> MAASGLDHLKNGYRRRFCRPSRARDINTEQGQNVLEILQDCFEEKSLANDFSTNSTKSVPNSTRKIKDTCIQSPSKECQKSHPKSVPVSSKKKEASLQFVVEPSEATNRSVQAHEVHQKILATDVS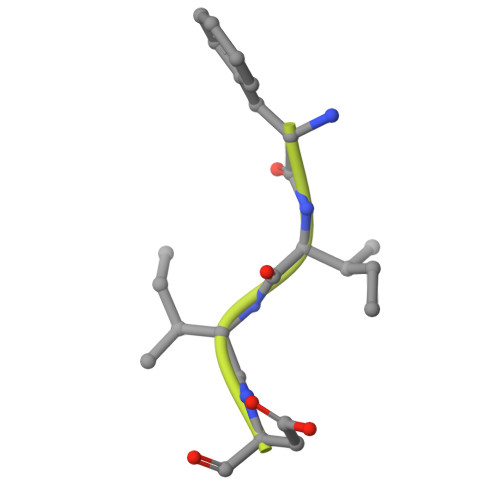SKNTPDSKKISSRNINDHHSEADEEFYLSVGSPSVLLDAKTSVSQNVIPSSAQKRETYTFENSVNMLPSSTEVSVKTKKRLNFDDKVMLKKIEIDNKVSDEEDKTSEGQERKPSGSSQNRIRDSEYEIQRQAKKSFSTLFLETVKRKSESSPIVRHAATAPPHSCPPDDTKLIEDEFIIDESDQSFASRSWITIPRKAGSLKQRTISPAESTALLQGRKSREKHHNILPKTLANDKHSHKPHPVETSQPSDKTVLDTSYALIGETVNNYRSTKYEMYSKNAEKPSRSKRTIKQKQRRKFMAKPAEEQLDVGQSKDENIHTSHITQDEFQRNSDRNMEEHEEMGNDCVSKKQMPPVGSKKSSTRKDKEESKKKRFSSESKNKLVPEEVTSTVTKSRRISRRPSDWWVVKSEESPVYSNS6-(3-aminopropyl)-4-(3-hydroxyphenyl)-9-(1H-pyrazol-4-yl)benzo[h]isoquinolin-1(2H)-one 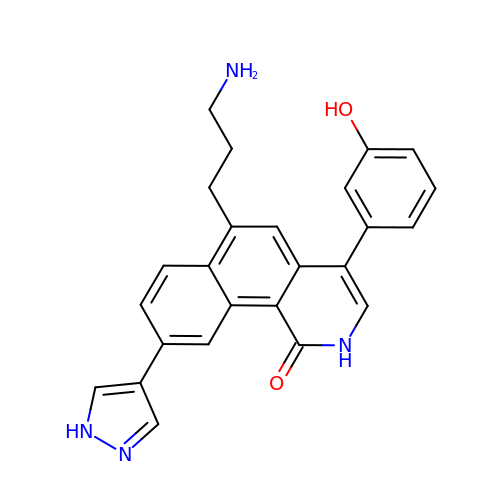| C25 H22 N4 O2 | BUSJQQYKXHYDNN-UHFFFAOYSA-N>MARKYFVAANWKCNGTLESIKSLTNSFNNLDFDPSKLDVVVFPVSVHYDHTRKLLQSKFSTGIQNVSKFGNGSYTGEVSAEIAKDLNIEYVIIGHFERRKYFHETDEDVREKLQASLKNNLKAVVAFGESLEQREQNKTIEVITKQVKAFVDLIDNFDNVILVYEPLWAIGTGKTATPEQAQLVHKEIRKIVKDTCGEKQANQIRILYGGSVNTENCSSLI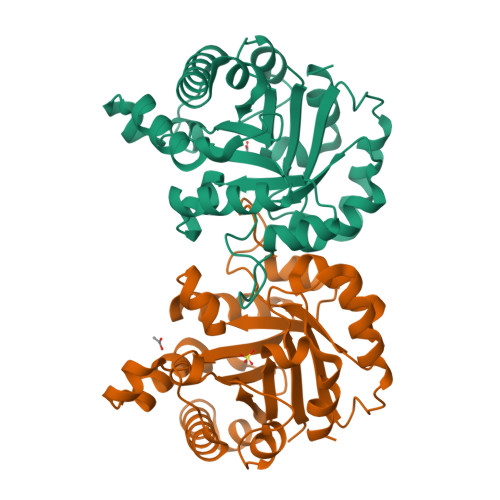QQEDIDGFLVGNASLKESFVDIIKSAM[2x]> MKIQAGQLGLDDNDVPGPLPDTDSKPSSQSQNDTPMFKLGNFESPVLKELSRRTVNKEMETQRIMTNVIAFAFWNLLVKFIKFFWNNTHVGRQFCNRLSRIHLYMLTFHTLKKANIIYHTTFSWLNAELLDYLFHLLISLNILFSLWKLLSTVKVSDLNLTDRQKKLLGVDMQSSVDTGLQPQHPHYVSTSKISQMAQNKTHIPQTNLKNH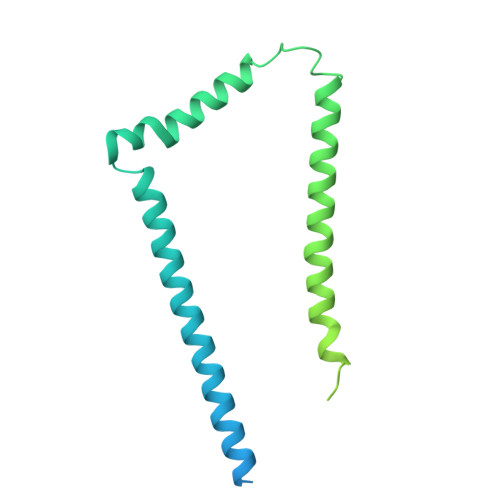PAYLFKGLETPLKARQREMAEEQTKLQSQSLHTKNVFGTLQRHSGISSTLVSANNDNNSPHTPVTRKGYIPSSKYAYMMNSQSPRGKI> HGTQGFAVLSYVYEHEKRDLASRIVSTQHHHHDLSVAT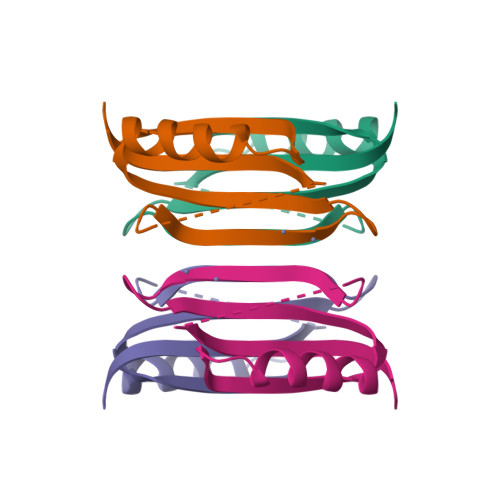LHVHINHDDCLEIAVLKGDMGDVQHFADDVIAQRGVRHGHLQCLPKED> LPTMNTPGSTQFLTSDDFQSPCALPQFDVTPSMNIPGEVKNLMEIAEVDSVVPVNNVQDTTDQMEMFRIPVTINAPLQQQVFGLRLQPGLDSVFKHTLLGEILNYYAHWSGSMKL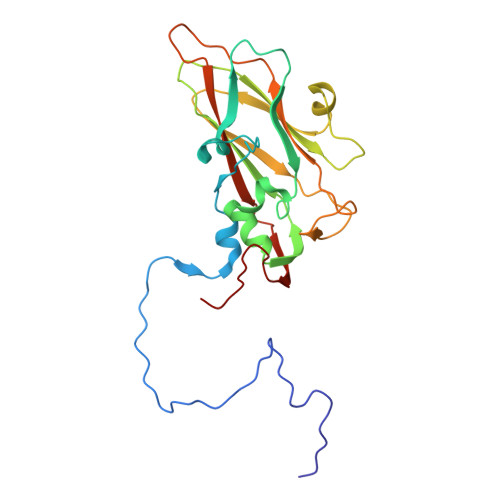TFVFCGSAMATGKFLIAYSPPGANPPKTRKDAMLGTHIIWDIGLQSSCVLCVPWISQTHYRLVQQDEYTSAGYVTCWYQTGMIVPPGTPNSSSIMCFASACNDFSVRMLRDTPFISQDNKL> MHHHHHHMGLNTAIATRVNGTPPPEVPIADIELGSLDFWALDDDVRDGAFATLRREAPISFWPTIELPGFVTGNGHWALTKYDDVFYASRHPDIFSSYPNITINDQTPELAEYFGSMIVLDDPRHQRLRSIVSRAFTPKVVARIEAAVRDRAHRLVSSMIANNPDRQADLVSELAGPLPLQIICDMMGIPKADHQRIFHWTN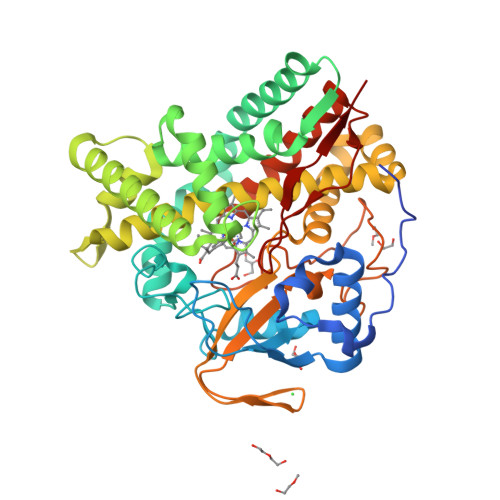VILGFGDPDLATDFDEFMQVSADIGAYATALAEDRRVNHHDDLTSSLVEAEVDGERLSSREIASFFILLVVAGNETTRNAITHGVLALSRYPEQRDRWWSDFDGLAPTAVEEIVRWASPVVYMRRTLTQDIELRGTKMAAGDKVSLWYCSANRDESKFADPWTFDLARNPNPHLGFGGGGAHFCLGANLARREIRVAFDELRRQMPDVVATEEPARLLSQFIHGIKTLPVTWS> QAQITGRPEWIWLALGTALMGLGTLYFLVKGMGVSDPDAKKFYAITTLVPAIAFTMYLSMLLGYGLTMVPFGGEQNP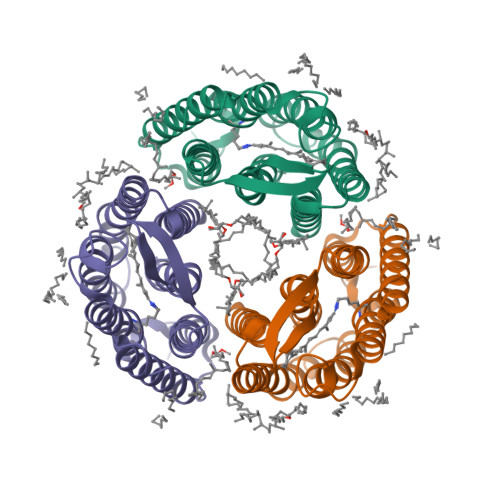IYWARYADWLFTTPLLLLDLALLVDADQGTILALVGADGIMIGTGLVGALTKVYSYRFVWWAISTAAMLYILYVLFFGFTSKAESMRPEVASTFKVLRNVTVVLWSAYPVVWLIGSEGAGIVPLNIETLLFMVLDVSAKVGFGLILLRSRAIFGEAE> DASIATFKGSEYFCYDLSQNPIQSSSDEITLSFKTLQRNGLM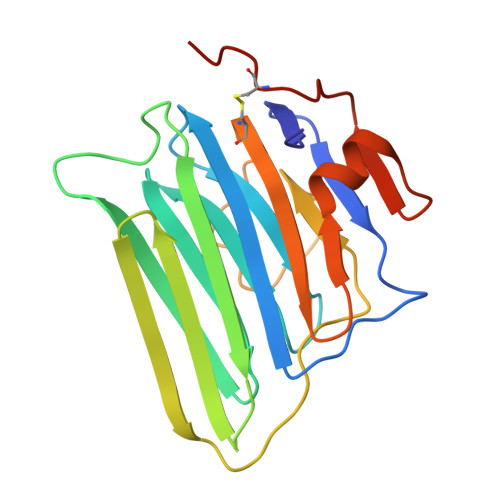LHTGKSADYVNLALKNGAVSLVINLGSGAFEALVEPVNGKFNDNAWHDVKVTRNLRQHSGIGHAMVTISVDGILTTTGYTQEDYTMLGSDDFFYVGGSPSTADLPGSPVSNNFMGCLKEVVYKNNDVRLELSRLAKQGDPKMKIHGVVAFKCAALEVLFQ4'-methylthymidine 5'-(tetrahydrogen triphosphate) | C11 H19 N2 O14 P3 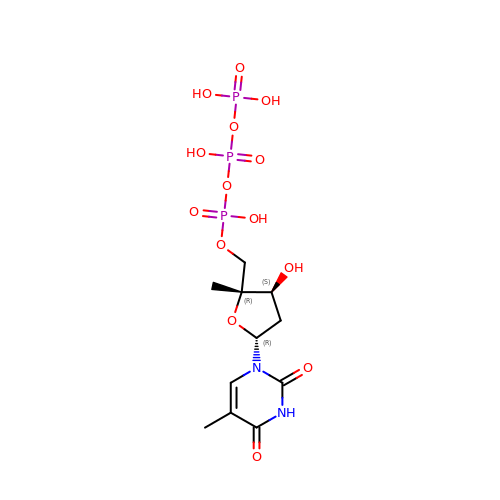| IUVOCYKHODEDJI-VAOFZXAKSA-N>MKLTPKELDKLMLHYAGELAKKRKEKGIKLNYVEAVALISAHIMEEARAGKKTAAELMQEGRTLLKPDDVMDGVASMIHEVGIEAMFPDGTKLVTVHTPIEANGKLVPGELFLKNEDITINEGKKAVSVKVKNVGDRPVQIGSHFHFFEVNRCLDFDREKTFGKRLDIASGTAVRFEPGEEKSVELIDIGGNRRIFGFNALVDRQADNESKKIALHRAKERGFHGAKSDDNYVKTIKE[12x];>[12x]MKKISRKEYVSMYGPTTGDKVRLGDTDLIAEVEHDYTIYGEELKFGGGKTLREGMSQSNNPSKEELDLIITNALIVDYTGIYKADIGIKDGKIAGIGKGGNKDMQDGVKNNLSVGPATEALAGEGLIVTAGGIDTHIHFISPQQIPTAFASGVTTMIGGGTGPADGTNATTITPGRRNLKWMLRAAEEYSMNLGFLAKGNASNDASLADQIEAGAIGFKIHEDWGTTPSAINHALDVADKYDVQVAIHTDTLNEAGCVEDTMAAIAGRTMHTFHTEGAGGGHAPDIIKVAGEHNILPASTNPTIPFTVNTEAEHMDMLMVCHHLDKSIKEDVQFADSRIRPQTIAAEDTLHDMGIFSITSSDSQAMGRVGEVITRTWQTADKNKKEFGRLKEEKGDNDNFRIKRYLSKYTINPAIAHGISEYVGSVEVGKVADLVLWSPAFFGVKPNMIIKGGFIALSQMGDANASIPTPQPVYYREMFAHHGKAKYDANITFVSQAAYDKGIKEELGLERQVLPVKNCRNITKKDMQFNDTTAHIEVNPETYHVFVDGKEVTSKPANKVSLAQLFSIF;>MNTYAQESKLRLKTKIGADGRCVIEDNFFTPPFKLMAPFYPKDDLAEIMLLAVSPGMMRGDAQDVQLNIGPNCKLRITSQSFEKIHNTEDGFASRDMHIVVGENAFLDFAPFPLIPFENAHFKGNTTISLRSSSQLLYSAIIVAGRVARNELFKFNRLHTKISILQDEKPIYYDNTILDPKTTDLNNMCMFDGYTHYLNLVLVNCPIELSGVRECIEESEGVDGAVSETASSHLCVKALAKGSEPLLHLREKIARLVTQTTTQKVWSHPQFEK[12x];>MDKGKSVKSTEKSVGMPPKTPKTDNNAHVDNEFLILQVNDAVFPIGSYTHSFGLETYIQQKKVTNKESALEYLKANLSSQFLYTEMLSLKLTYESALQQDLKKILGVEEVIMLSTSPMELRLANQKLGNRFIKTLQAMNELDMGEFFNAYAQKTKDPTHATSYGVFAASLGIELKKALAHYLDAQTSNMVINCVKSVPLSQNDGQKILLSLQSPFNQLIEKTLELDESHLCTASVQNDIKAMQHESLYSRLYMS[12x]

Urease is a nickel (Ni) enzyme that is essential for the colonization of Helicobacter pylori in the human stomach. Ni delivery requires urease to form an activation complex with the urease accessory proteins UreFD and UreG. Here, we determined the cryo–electron microscopy structures of H. pylori UreFD/urease and Klebsiella pneumoniae UreD/urease complexes at 2.3- and 2.7-angstrom resolutions, respectively. Combining structural, mutagenesis, and biochemical studies, we show that the formation of the activation complex opens a 100-angstrom-long tunnel, where the Ni ion is delivered through UreFD to the active site of urease.

Here, we introduced R179A/Y183D substitutions to HpUreF so that we could obtain discrete particles of HpUreFD/urease complexes for cryo-EM analyses. Additional substitution of E140A to HpUreD was found to stabilize the complex, and protein samples of H. pylori urease (HpUreAB) in complex with HpUreF(R179A/Y183D) and HpUreD(E140A) were finally used for data collection. Four copies of the urease trimers form a dodecameric quaternary structure with 12 protruding HpUreFD molecules. As expected, the R179A/Y183D substitutions disrupted the dimerization of HpUreFD, and each catalytic unit of H. pylori urease is interacting with one copy of HpUreD and HpUreF. Binding of UreD induces major conformational changes in three switch regions of HpUreB: (i) the glycine-rich loop (277GAGGGHAP284) between strand 6 and helix 6, (ii) helix H3 and the loop connecting to helix 7 (residues 330 to 340), and (iii) residues between strand 12 and strand 13 (residues 538 to 545). Upon binding of HpUreFD, residues 335ADSR338 at the C terminus of helix H3 uncoil, causing switches II and III residues to stretch in opposite directions and residues Arg338 and Arg340 to flip out toward UreD. The stretching motion of helix H3 brings Val332 of HpUreB to dock into a hydrophobic pocket of HpUreD formed by Met36, Phe39, Met49, and Leu51. We noticed that the formation of the HpUreFD/urease complex opens a tunnel that reaches the active site of urease. Tunnel searching was performed using the program CAVER 3.0 (22). This 100-Å-long tunnel starts at the active site residue Lys219 of urease, exits HpUreB near Asp336 of the switch II region, passes through HpUreD between the two layers of β sheets, enters HpUreF near Ala233, and reaches the dimerization interface of HpUreF. The UreD/urease interaction causes Phe112 to flip to an exposed position and thereby open a passage that connects the tunnel between HpUreB and HpUreD.> MCDLRKTKLIDKISSLELYKYSIFFRNYIENVAEDCLKNGLILESAAHNVSEVELARLKVQLKNALLNCIISYRFHGIGYVLVKTKDTLIDLEQPVNIELPIGFEYLDYEYVRDLGVDFDHITYKVKSNNKNNSLDAVKIHKSRLIIYENFDYILKRYVPCYTESFLLDIYLFEKIYVEIERRIENHNFLFYKDESLVQLQDALSSATTSLSALTQSNNDRGSGILSSFLRKQNSNNHSKDISNLRNLNDSLSQELARLKSNLNNEGMFYTATPSASLEVIKYDLSYLKEALALIKAKIGADTKEPLTRSFNEQAKGLGNDGKGDRSNYYDFLKGVQEQVENSCNLKLTKYFGLDMKFNSLIMLSEEQKVERDIKLIELYSKYNQLIQSSSFNNEELAMLKEKLFSF;> MTEKEEKE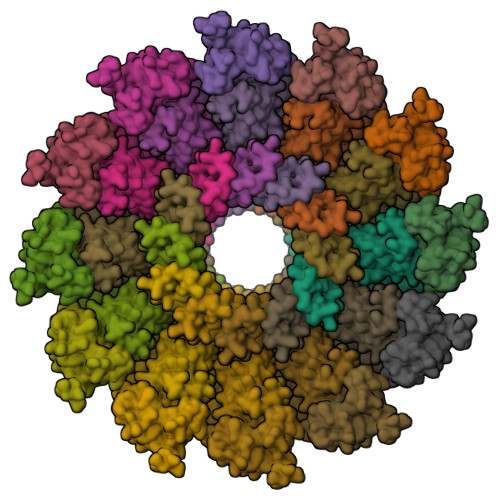DLQAQDKEEQQIKADTKVISVQEFEEYMRFKEQANSKSKETSRDLSINERITKELAEVEERERIEKQLLLEAERINEIDTLAKAHLSNHFNKEVLLAKGYTLKDIMQAQRRELVRKFVPIEQIKAIAKVSDISHIDGEILEQLVSLAKVNIKLRKNASSSSSSVDSIKGNIAIKSEERASLLDSNFVPINFTEFVQAISNTYKQRRIQFYENLKRHKRTSIA>IQTTAPPVKESSFVEKMKKTGRNIIVFYGSQTGTAEEFANRLSKDAHRYGMRGMSADPEEYDLADLSSLPEIDKSLVVFCMATYNGDPTDNAQDFYDWLQETDVDLTGVKFAVFGLGNKTYEHFNAMGKYVDQRLEQLGAQRIFELGLGDDDGNLEEDFITWREQFWPAVCEFFGVEATGEESSIRQYELVVHEDMDVAKVYTGEMGRLKSYENQKPPFDAKNPFLAAVTANRKLNQGTERHLMHLELDISDSKIRYESGDHVAVYPANDSALVNQIGEILGADLDVIMSLNNLDEESNKKHPFPCPTTYRTALTYYLDITNPPRTNVLYELAQYASEPSEQEHLHKMASSSGEGKELYLSWVVEARRHILAILQDYPSLRPPIDHLCELLPRLQARYYSIASSSKVHPNSVHICAVAVEYEAKSGRVNKGVATSWLRAKEPAGENGGRALVPMFVRKSQFRLPFKSTTPVIMVGPGTGIAPFMGFIQERAWLREQGKEVGETLLYYGCRRSD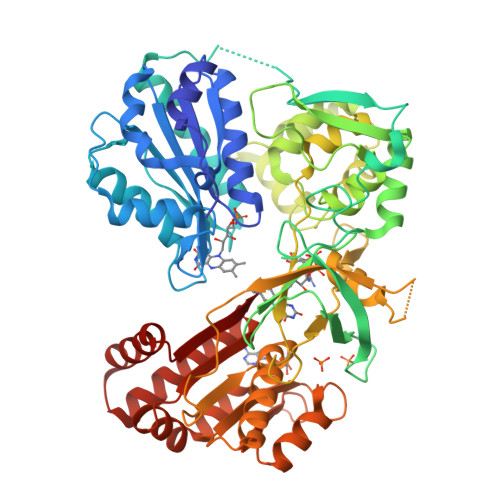EDYLYREELARFHKDGALTQLNVAFSREQAHKVYVQHLLKRDREHLWKLIHEGGAHIYVCGDARNMAKDVQNTFYDIVAEFGPMEHTQAVDYVKKLMTKGRYSLDVWS[2x]>[2x]MALKQISSNKCFGGLQKVFEHDSVELNCKMKFAVYLPPKAETGKCPALYWLSGLTCTEQNFISKSGYHQSASEHGLVVIAPDTSPRGCNIKGEDESWDFGTGAGFYVDATEDPWKTNYRMYSYVTEE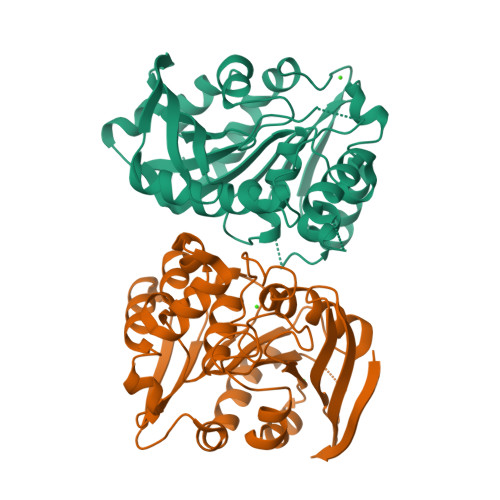LPQLINANFPVDPQRMSIFGHSMGGHGALICALKNPGKYKSVSAFAPICNPVLCPWGKKAFSGYLGTDQSKWKAYDATHLVKSYPGSQLDILIDQGKDDQFLLDGQLLPDNFIAACTEKKIPVVFRLQEDYDHSYYFIATFITDHIRHHAKYLNA>MGEVNKDAVEKYLENNPQFAKEYFDRKMRAEVLGSIFQVSPGDVKEGVSFKDMSRLEECNILFELLTEIQDEAGSMEKIVHKTLQRLSQLLARDRCSMFICRSRNGIPEVATRLLNVTPTSKFEDNLVNPDKETVFPLDIGIAGWVAHTKKFFNIPDVKKNNHFSDYLDKKTGYTTVNMMAIPITQGKEVLAVVMALNKLNASEFSKEDEEVFKKYLNFISLVLRNHHTSYLYNIESRRSQMLLWSANKVFEELTDIERQFHKALYTIRMYLNCERYSVGLLDMTKEKEFYDEWPIRLGEAEPYKGPKTPDGREVNFYKIIDYILHGKEEIKVIPTPPADHWCLISGLPTYVAENGFICNMMNAPADEYFTFQKGPVDETGWVIKNVLSLPIVNKKEEIVGVATFYNRKDGKPFDEYDEQIIETLTQFLGWSVLNTDTYDKMNKLENRKDIAQEMLMYQTKATPTEVESILKYKEKLNVKSIEECDEKDLIRILKEELPDPKDLELYEFRFSDFPVTEHGLITCGIRLFFEINVVEKFKVPAEVLTRWMYTVRKGYRDITYHNWRHGFNVGQTMFTLLMTGRIKKYYTDLEAFAMVAAAFCHDIDHRGTNNLYQMKSAAPLAKLHGSSILERHHLEYSKTLLQDESLNIFQNLNKRQFETVLHLFEVAIIATDLALYFKKRTMFQKIVDAIEKMETEEEAIKYISIDPTKKE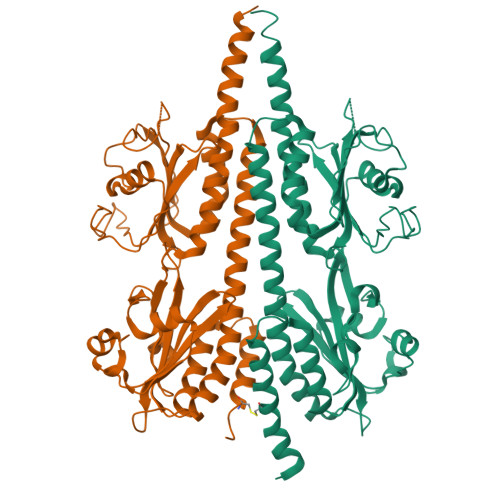VIMAMMMTGCDLSAITKPWEVQSKVALMVANEFWEQGDLERTVLQQQPIPMMDRNKGDELPKLQVGFIDFVCTFVYKEFSRFHKEITPMFDGLQNNRVEWKTRADEYEEKMKVIEEQKKKEEEAAAKKAENAAGGGGGGEDGKSKTCIVL[2x]> MNALHRIGAGTLLAVLLAFGLTGCGEKEEVQQSLEPVAFHDSDECHVCGMIITDFPGPKGQAVEKRGV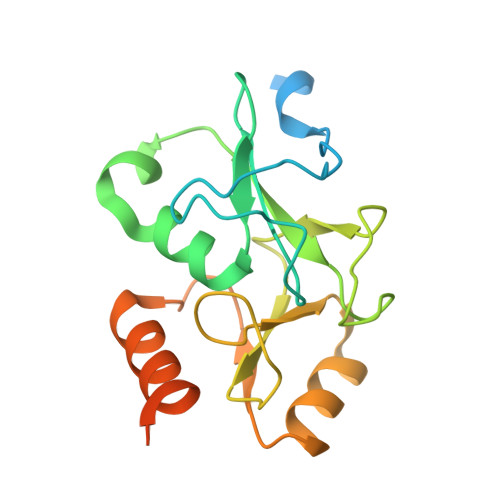KKFCSTAEMLGWWLQPENRLLDAKLYVHDMGRSVWEKPDDGHLIDATSAYYVVGTSLKGAMGASLASFAEEQDAKALAGMHGGRVLRFEEIDQALLQEAASMQHGGMHDHAPNGAHNAHAGHWSHPQFEK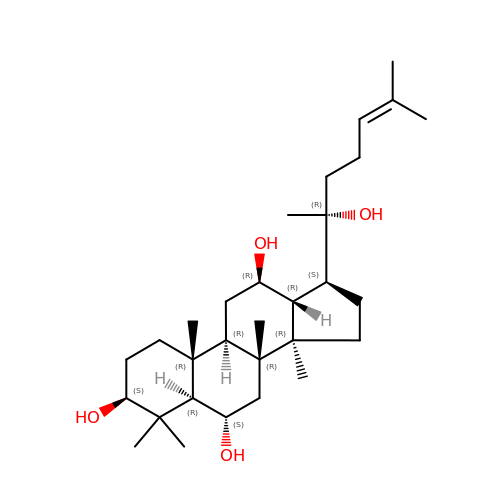(3S,5R,6S,8R,9R,10R,12R,13R,14R,17S)-4,4,8,10,14-pentamethyl-17-[(2R)-6-methyl-2-oxidanyl-hept-5-en-2-yl]-2,3,5,6,7,9,11,12,13,15,16,17-dodecahydro-1H-cyclopenta[a]phenanthrene-3,6,12-triol | C30 H52 O4 | SHCBCKBYTHZQGZ-DLHMIPLTSA-N>MGRIKNKQFAVIGLGKFGGSICKELHRMGHEVLAVDINEEKVNAYASYATHAVIANATEENELLSLGIRNFEYVIVAIGANIQASTLTTLLLKELDIPNIWVKAQNYYHHKVLEKIGADRIIHPEKDMGVKIAQSLSDENVLNYIDLSDEYSIVELLATRKLDSKSIIDLNVRAKYGCTILAIKHHGDICLSPAPEDII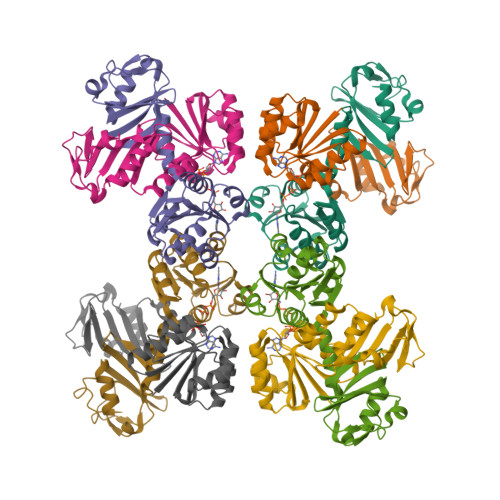REQDCLVIMGHKKDIKRFENEGM[8x]>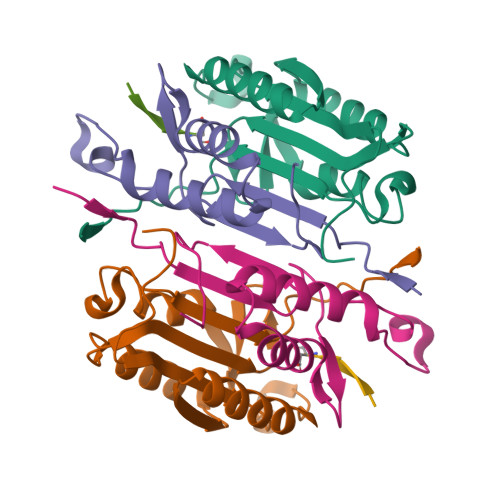[2x]DNSYKMDYPEMGLCIIINNKNFHKSTGMTSRSGTDVDAANLRETFRNLKYEVRNKNDLTREEIVELMRDVSKEDHSKRSSFVCVLLSHGEEGIIFGTNGPVDLKKITNFFRGDRCRSLTGKPKLFIIQACRGTELDCGIET;>CHKIPVEADFLYAYSTAPGYYSWRNSKDGSWFIQSLCAMLKQYADKLEFMHILTRVNRKVATEFESFSFDATFHAKKQIPCIVSMLTKELYFYHH[2x];>[2x]XVDRVD> MGHHHHHHENLYFQGMADAWEEIRRLAADFQRAQFAEATQRLSERNCIEIVNKLIAQKQLEVVHTLDGKEYITPAQISKEMRDELHVRGGRVNIVDLQQVINVDLIHIENRIGDIIKSEKHV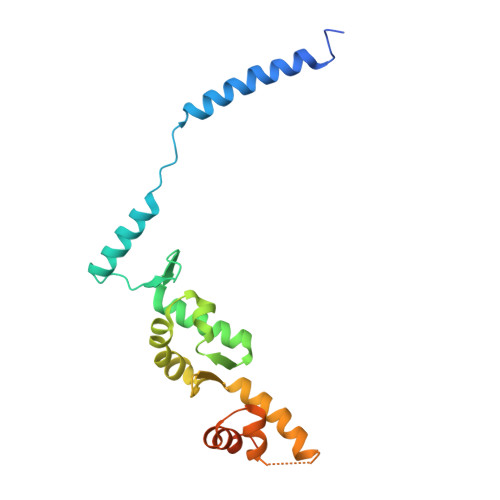QLVLGQLIDENYLDRLAEEVNDKLQESGQVTISELCKTYDLPGNFLTQALTQRLGRIISGHIDLDNRGVIFT> MVSFFKTPIFILIIFLYLNEKVICSINENQNENDTISQNVNQHENINQNVNDNDNIEQLKSMIGNDELHKNLTILEKLILESLEKDKLKYPLLKQGTEQLIDISKFNKKNITDADDETYIIPTVQSTFHDIVKYEHLIKEQSIEIYNSDISDKIKKKIFIVRTLKTIKLMLIPLNSYKQNNDLKSALEELNNVFTNKEAQEESSPIGDHGTFFRKLLTHVRTIKENEDIENKGETLILGDNKIDVMNSNDFFFTTNSNVKFMENLDDITNQYGLGLINHLGPHLIALGHFTVLKLALKNYKNYFEAKSIKFFSWQKILEFSMSDRFKVLDMMCDHESVYYSEKKRRKTYLKVDRSNTSMECNILEYLLHYFNKYQLEIIKTTQDTDFDLHGMMEHKYIKDYFFSFMCNDPKECIIYHTNQFKKEANEENTFPEQEEPNRQISAFNLYLNYYYFMKRYSSYGVKKTLYVHLLNLTGLLNYDTRAYVTSLYLPGYYNAVEMSFTEEKEFSKLFESLIQCIEKCHSDQARQISKDSNLLNNITKCDLCKGAFLYANMKFDEVPSMLQKFYVYLTKGLKIQKVSSLIKTLDIYQDYSNYLSHDINWYTFLFLFRLTSFKEIAKKNVAEAMYLNIKDEDTFNKTVVTNYWYPSPIKKYYTLYVRKHIPNNLVDELEKLMKSGTLEKMKKSLTFLVHVNSFLQLDFFHQLNEPPLGLPRSYPLSLVLEHKFKEWMNSSPAGFYFSNYQNPYIRKDLHDKVLSQKFEPPKMNQWNKVLKSLIECAYDMYFEQRHVKNLYKYHNIYNINNKLMLMRDSIDLYKNNFDDVLFFADIFNMRKYMTATPVYKKVKDRVYHTLHSITGNSVNFYKYGIIYGFKVNKEILKEVVDELYSIYNFNTDIFTDTSFLQTVYLLFRRIEETYRTQRRDDKISVNNVFFMNVANNYSKLNKEEREIEIHNSMASRYYAKTMFAAFQMLFSTMLSNNVDNLDKAYGLSENIQVATSTSAFLTFAYVYNGSIMDSVTNSLLPPYAKKPITQLKYGKTFVFSNYFMLASKMYDMLNYKNLSLLCEYQAVASANFYSAKKVGQFLGRKFLPITTYFLVMRISWTHAFTTGQHLISAFGSPSSTANGKSNASGYKSPESFFFTHGLAAEASKYLFFYFFTNLYLDAYKSFPGGFGPAIKEQTQHVQEQTYERKPSVHSFNRNFFMELVNGFMYAFCFFAISQMYAYFENINFYITSNFRFLDRYYGVFNKYFINYAIIKLKEITSDLLIKYEREAYLSMKKYGYLGEVIAARLSPKDKIMNYVHETNEDIMSNLRRYDMENAFKNKMSTYVDDFAFFDDCGKNEQFLNERCDYCPVIEEVEETQLFTTTGDKNTNKTTEIKKQTSTYIDTEKMNEADSADSDDEKDSDTPDDELMISRFH;> MIKVTIFLLLSIFSFNLYGLELNEKVSIKYGAEQGVGSADSNTKLCSDILKYLYMDEYLSEGDKATFEKKCHNVIGNIRNTFSNKNTIKEGNEFLMSILHMKSLYGNNNNNNAGSESDVTLKSLYLSLKGSQNTEGESEVPSDDEINKTIMNFVKFNKYLLDNSNDIKKVHDFLVLTSQSNENLLPNKEKLFEQIVDQIKYFDEYFFASGGKIKVKKGYLKYNFLDIYKQPVCSAYLHLCSRYYESVSIYIRLKKVFNGIPAFLDKNCRKVKGEEFKKLMDMELKHNHIVERFDKYIISDDLYYVNMKVFDLKNVDKIQVSKIDDINNLNIYEHKETMHLSAKNLSRYIDIKKELNDEKAYKQLMSAIRKYVTTLTKADSDITYFVKQLDDEEIERFLIDLNFFLYNGFLRITEDKHLINADDVSPSYINLYRSNNIVALYILKTQYEENKLSEYRAHKFYRRKRVSNITNDMIKKDFTQTNALTNLPNLDNKKTTEYYLKEYENFVENFQPDLHDIMKLQLFFTMAFKDCNVNQNFTETSKKLWFDLLYAYDKFGWFYIHPNEVINSINKTDFVRHVLVSRNFLLKNNDQLTFLETQVAKIVEIINLSLEVDKSPDSLDFSIPMNFFNHKNGYHVMNDDKLKLLTSYEYIDSIANNYFFLSEYKNDVFRTGNNFKLYFNLPNIYSLAYQLFNELAININVITNVPLKKYLKYNASYAYFTLMNMIGKNHDIYSKGSRFVYASYILGLVFFIESHIDIARLKPKDFFFMKQSLPIIDHVYHKDLKTLKKNCTLLTDFMKINKNSQNYSLTHTEEMIKILGLLTVTLWAKEGKKSVYYDDDVSLYRKLMVSCVFNGGETIQEKLANNIEKSCDISQYGIKSKNLKDMIDINLSIHKWNPAEIEKLAYSFVLSCKMQKLMYKPMNVEKLPLEDYYKLSLAPDMVKTYHCYKLGKQAAELLESIILKKKFVRFRVTDAIDVYDFFYIKKVLSSRIKKEYNEFLQDKRAFEKKELETILNNSPFSEEQTMKLINSYECHWFTSYENFRILWMHASSNLGTGTYLKNFFSELWQNIRFLFKSKLKIRDMEYFSGDISQMNLLDYYSPMVHSESHCQEKMQVLFITLRDSKEENRSEIAQKVKSAYYQCKLDYYKNHHSDFIHRIHPNDFLNNKVYVLKQPYYLMSNVPLNNPKKVSRLFVTEGTLEYLLLDKINIPECFGPCTKLHFNKVVIKESKQRIYDMTINNALVPEIQPYNRRKYMTIYINEAYIKNIVSDALTSEEIKRHDIQKGNIKICMGKSTYLTEPILTEEHFNLTHKPVYDFSSVKHNLKVFHMKNEHLVSEDPNDDCFINYPLATINLDISDPYKEISEDLIKNLYILKSS;> MRSKHLVTLFIITFLSFSTVKVWGKDVFAGFVTKKLKTLLDCNFALYYNFKGNGPDAGSFLDFVDEPEQFYWFVEHFLSVKFRVPKHLKDKNIHNFTPCLNRSWVSEFLKEYEEPFVNPVMKFLDKEQRLFFTYNFGDVEPQGKYTYFPVKEFHKYCILPPLIKTNIKDGESGEFLKYQLNKEEYKVFLSSVGSQMTAIKNLYSTVEDEQRKQLLKVIIENESTNDISVQCPTYNIKLHYTKECANSNNILKCIDEFLRKTCEKKTESKHPSADLCEHLQFLFESLKNPYLDNFKKFMTNSDFTLIKPQSVWNVPIFDIYKPKNYLDSVQNLDTECFKKLNSKNLIFLSFHDDIPNNPYYNVELQEIVKLSTYTYSIFDKLYNFFFVFKKSGAPISPVSVKELSHNITDFSFKEDNSEIQC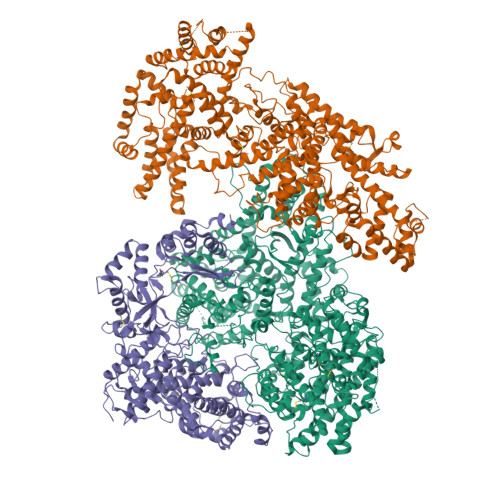QNVRKSLDLEVDVETMKGIAAEKLCKIIEKFILTKDDASKPEKSDIHRGFRILCILISTHVEAYNIVRQLLNMESMISLTRYTSLYIHKFFKSVTLLKGNFLYKNNKAIRYSRACSKASLHVPSVLYRRNIYIPETFLSLYLGLSNLVSSNPSSPFFEYAIIEFLVTYYNKGSEKFVLYFISIISVLYINEYYYEQLSCFYPKEFELIKSRMIHPNIVDRILKGIDNLMKSTRYDKMRTMYLDFESSDIFSREKVFTALYNFDSFIKTNEQLKKKNLEEISEIPVQLETSNDGIGYRKQDVLYETDKPQTMDEASYEETVDEDAHHVNEKQHSAHFLDAIAEKDILEEKTKDQDLEIELYKYMGPLKEQSKSTSAASTSDEISGSEGPSTESTSTGNQGEDKTTDNTYKEMEELEEAEGTSNLKKGLEFYKSSLKLDQLDKEKPKKKKSKRKKKRDSSSDRILLEESKTFTSENEL>SMHSDLTFCEIILMEMESHDAAWPFLEPVNPRLVSGYRRIIKNPMDFSTMRHRLSRGGYTSSEEFAADALLVFDNCQTFNEDDSEVGKAGHIMRR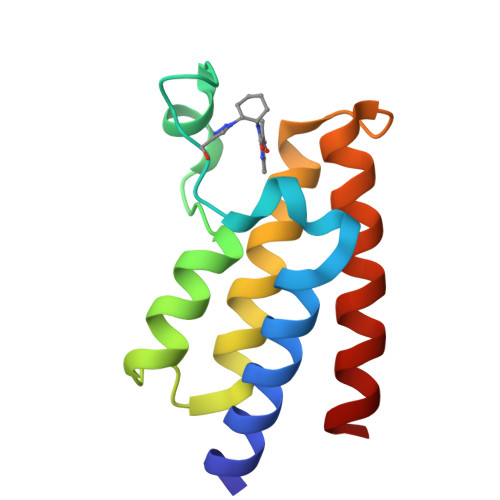FFESRWEEFYQ[3x]> MKRNYILGLDIGITSVGYGIIDYETRDVIDAGVRLFKEANVENNEGRRSKRGARRLKRRRRHRIQRVKKLLFDYNLLTDHSELS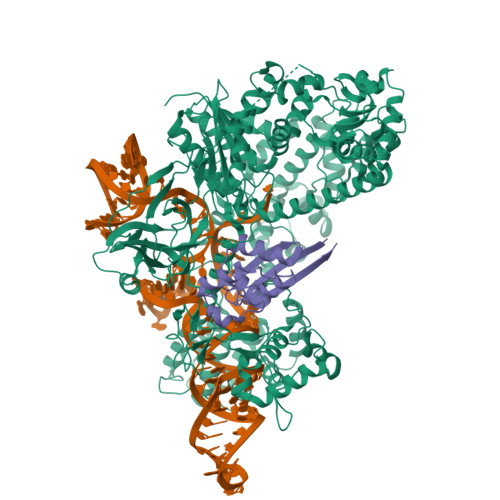GINPYEARVKGLSQKLSEEEFSAALLHLAKRRGVHNVNEVEEDTGNELSTKEQISRNSKALEEKYVAELQLERLKKDGEVRGSINRFKTSDYVKEAKQLLKVQKAYHQLDQSFIDTYIDLLETRRTYYEGPGEGSPFGWKDIKEWYEMLMGHCTYFPEELRSVKYAYNADLYNALNDLNNLVITRDENEKLEYYEKFQIIENVFKQKKKPTLKQIAKEILVNEEDIKGYRVTSTGKPEFTNLKVYHDIKDITARKEIIENAELLDQIAKILTIYQSSEDIQEELTNLNSELTQEEIEQISNLKGYTGTHNLSLKAINLILDELWHTNDNQIAIFNRLKLVPKKVDLSQQKEIPTTLVDDFILSPVVKRSFIQSIKVINAIIKKYGLPNDIIIELAREKNSKDAQKMINEMQKRNRQTNERIEEIIRTTGKENAKYLIEKIKLHDMQEGKCLYSLEAIPLEDLLNNPFNYEVDHIIPRSVSFDNSFNNKVLVKQEENSKKGNRTPFQYLSSSDSKISYETFKKHILNLAKGKGRISKTKKEYLLEERDINRFSVQKDFINRNLVDTRYATRGLMNLLRSYFRVNNLDVKVKSINGGFTSFLRRKWKFKKERNKGYKHHAEDALIIANADFIFKEWKKLDKAKKVMENQMFEEKQAESMPEIETEQEYKEIFITPHQIKHIKDFKDYKYSHRVDKKPNRELINDTLYSTRKDDKGNTLIVNNLNGLYDKDNDKLKKLINKSPEKLLMYHHDPQTYQKLKLIMEQYGDEKNPLYKYYEETGNYLTKYSKKDNGPVIKKIKYYGNKLNAHLDITDDYPNSRNKVVKLSLKPYRFDVYLDNGVYKFVTVKNLDVIKKENYYEVNSKCYEEAKKLKKISNQAEFIASFYNNDLIKINGELYRVIGVNNDLLNRIEVNMIDITYREYLENMNDKRPPRIIKTIASKTQSIKKYSTDILGNLYEVKSKKHPQIIKKG;> MEKVDTWIVYRGRTADMNKSYIAEGSTYEEVYNNFVDKYGYDVLDEDIYEIQLLKKNGENLDDYDVDSDGINNYDKLDEFRESDYVDLEDYDYRELFENSSSQVYYHEFEITHE> TAYYAQALQSVPETQVSQLDNGVRVASEQSSQPTCTVGVWIDAGSRYESEKNNGAGYFLEHLAFKGTKNRPQNALEKEVESMGAHLNAYSSREHTAYYIKALSKDVPKAVELLADIVQNCSLEDSQIEKERDVIVRELQENDTSMREVVFNYLHATAFQGTGLAQSVEGPSENIRKLSRADLTEYLSTHYTAPRMVLAAAGGVEHQQLLELAQKHFGGVPFTYDDDAVPTLSKCRFTGSQIRHREDGLPLAHVAIAVEGPGWAHPDLVALQVANAIIGHYDRTYGGGLHSSSPLASIAVTNKLCQSFQTFSICYSETGLFGFYFVCDRMSIDDMMFVLQGQWMRLCTSISESEVLRGKNFLRNALVSHLDGTTPVCEDIGRELLTYGRRIPLEEWEERLAEVDARMVREVCSKYIYDQCPAVAGPGPIEQLPDYNRIRSGMFWLRF;> PPHPQDLEITKLPNGLVIASLENYSPGSTIGVFIKAGSRYENSSNLGTSHLLRLASSLTTKGASSFKITRGIEAVGGKLSVESTRENMAYTVECLRDDVEILMEFLLNVTTAPEFRPWEVADLQPQLKIDKAVAFQNPQTHVIENLHAAAYRNALADSLYCPDYRIGKVTSVELHDFVQNHFTSARMALVGLGVSHPVLKNVAEQLLNIRGGLGLSGAKAKYRGGEIREQNGDSLVHAAIVAESAAIGGAEANAFSVLQHVLGANPHVKRGLNATSSLYQAVAKGVHQPFDVSAFNASYSDSGLFGFYTISQAAYAGQVIKAAYNQVKT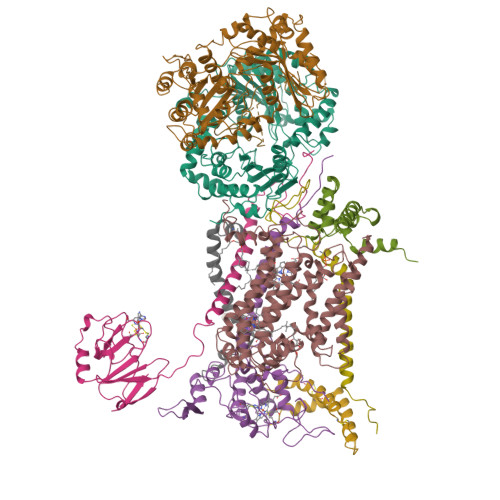IAQGNVSNENVQAAKNKLKAKYLMSVESSEGFLEEVGSQALAAGSYNPPSTVLQQIDAVADADVIKAAKKFVSRQKSMAASGNLGHTPFVDEL;> MAPNIRKSHPLLKMINNSLIDLPAPSNISAWWNFGSLLAVCLMTQILTGLLLAMHYTADTSLAFSSVAHTCRNVQYGWLIRNLHANGASFFFICIFLHIGRGLYYGSYLYKETWNTGVILLLTLMATAFVGYVLPWGQMSFWGATVITNLFSAIPYIGHTLVEWAWGGFSVDNPTLTRFFALHFLLPFAIAGITIIHLTFLHESGSNNPLGISSDSDKIPFHPYYSFKDILGLTLMLTPFLTLALFSPNLLGDPENFTPANPLVTPPHIKPEWYFLFAYAILRSIPNKLGGVLALAASVLILFLIPFLHKSKQRTMTFRPLSQTLFWLLVANLLILTWIGSQPVEHPFIIIGQMASLSYFTILLILFPTIGTLENKMLNY;> SDLELHPPSYPWSHRGPLSSLDHTSIRRGFQVYKQVCSSCHSMDYVAYRHLVGVCYTEDEAKALAEEVEVQDGPNEDGEMFMRPGKLSDYFPKPYPNPEAARAANNGALPPDLSYIVRARHGGEDYVFSLLTGYCEPPTGVSVREGLYFNPYFPGQAIGMAPPIYNDVLEFDDGTPATMSQVAKDVCTFLRWAAEPEHDHRKRMGLKMLLMMGLLVPLVYYMKRHKWSVLKSRKLAYRPPK;> SHTDIKVPNFSDYRRPPDDYSTKSSRESDPSRKGFSYLVTAVTTLGVAYAAKNVVTQFVSSMSASADVLAMSKIEIKLSDIPEGKNMAFKWRGKPLFVRHRTKKEIDQEAAVEVSQLRDPQHDLERVKKPEWVILIGVCTHLGCVPIANAGDFGGYYCPCHGSHYDASGRIRKGPAPLNLEVPSYEFTSDDMVIVG;> AGRPAVSASSRWLEGIRKWYYNAAGFNKYGLMRDDTIYENDDVKEAIRRLPENLYDDRMFRIKRALDLNMRQQILPKEQWTKYEEDVPYLEPYLKEVIRERKEREEWDK;> GRQFGHLTRVRHLITYSLSPFEQRPFPHYFSKGVPNVWRRLRACILRVAPPFLAFYLLYTWGTQEFEKSKRKNPAAYVNDR;> GDPKEEEEEEEELVDPLTTVREQCEQLEKCVKARERLELCDERVSSRSQTEEDCTEELFDFLHARDHCVAHKLFNSLK;> VAPTLTARLYSLLFRRTSTFALTIVVGALLFERAFDQGADAIYEHINEGKLWKHIKHKYENK>[2x]TVLP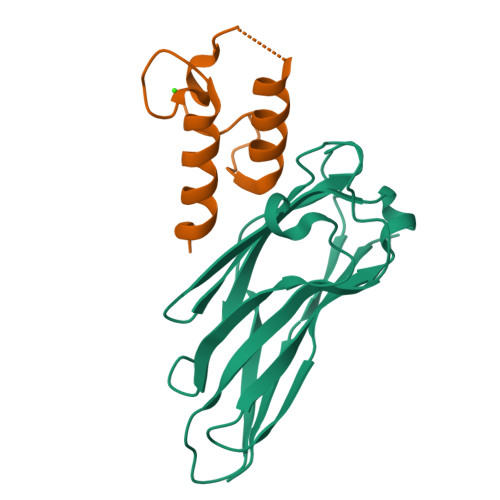KDIPGDSLKVTVGTANGKPGDTVTVPVTFADVAKMKNVGTCNFYLGYDASLLEVVSVDAGPIVKNAAVNFSSSASNGTISFLFLDNTITDELITADGVFANIKFKLKSVTAKTTTPVTFKDGGAFGDGTMSKIASVTKTNGSVTIDP;>[2x]VIVYGDYNNDGNVDALDFAGLKKYIMAADHAYVKNLDVNLDNEVNSTDLAILKKYLLGMVSKLPSN>GSHMQVWPGQAYPLGATYDGAGTNFAVFSEAAHRIELCLLHDDGSETAVELRETDAFVRHAYLPGVMPGQRYGFRVHGPYAPERGLRCNAAKLLLDPYARAVSGRVRWGEAVYGYPFGRPDARNDLDSAPDTMTSVVVNPYFDWGDDRRPRTEYHHTVIYEAHVKGLTMLHPDLPEELRGTYAGLAHPSVIGHLRELGVTALELMPVHQFVNDHRLVDAGLSNYWGYNTIGFFAPHNAYASWGDRGQQVLEFKSAVRALHQAGIEVILDVVYNHTAEGNHLGPTLSMRGLDNPSYYRLADDPRYYMDTTGTGNSLLMRSPHVLQLIMDSLRYWVTEMHVDGFRFDLAATLARQFHEVDRLSSFFDLVQQDPVVSQVKLIAEPWDVGEGGYQVGNFPPLWTEWNGKYRDCVRDLWRGEPRTLAEFASRLTGSSDLYQDDGRRPLASVNFVTCHDGFTLRDLVSYNEKRNEANGEGNRDGENYNRSWNCGEEGETEDVGITELRARQMRNFLATLMLSQGVPMLSHGDEFGRTQGGNNNAYCQDNEVSWV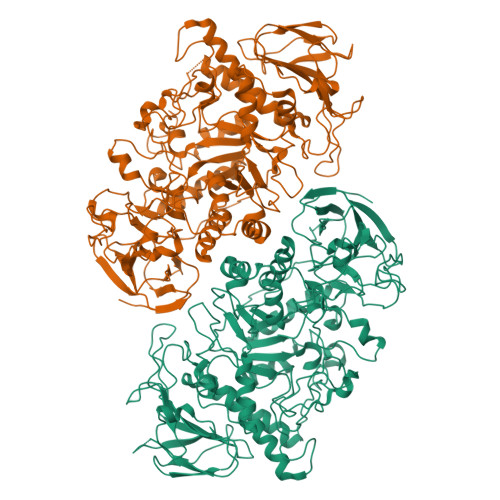RWPKENSEAEATLLRFTRSMVRLRREHPVFRRRRFFHGRPVEGTHDELTDIAWFTPEGEEMTSRDWQAAHAQALTVFLNGNAISEPGTQGERIADDSFLLMFNASAKELEFVVPDSHGRYWRMVVDTSDPEGMPPQQGPELAGGERVTLAPLSLTVLRRPA[12x]>[2x]WNIHGKESCDVQLYIKRQSEHSILAGDPFELECPVKYCANRPHVTWCKLNGTTCVKLEDRQTSWKEEKNISFFILHFEPVLPNDNGSYRCSANFQSNLIESHSTTLYVTDV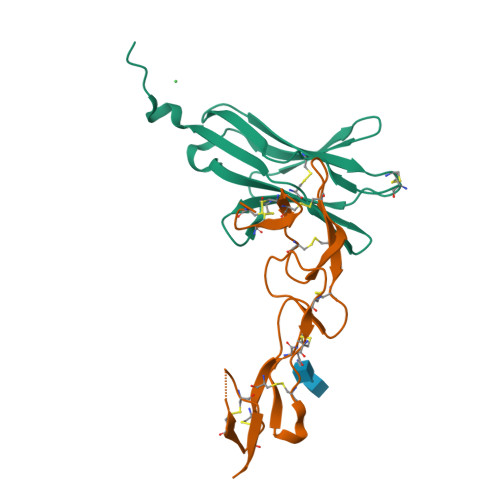KHHHHHHHH;>[2x]GSHMLPSCKEDEYPVGSECCPKCSPGYRVKEACGELTGTVCEPCPPGTYIAHLNGLSKCLQCQMCDPAMGLRASRNCSRTENAVCGCSPGHFCIVQDGDHCAACRAYA> GGAGCGUCGUGUCUCUUGUACGUCUCGGUCACAAUACACGGUUUCGUCCGGUGCGUGGCAAUUCGGGGCACAUCAUGUCUUUCGUGGCUGGUGUGACCGCGCAAGGUGCGCGCGGUACGUAUCGAGCAGCGCUCC

Stem-loop 5 (SL5, residues 150 to 294) contains the start codon of open reading frame 1a/b (ORF1a/b, residues 266 to 268). Additionally, phylogenetic covariance analysis and chemical probing experiments have shown that SL5′s secondary structure forms a four-way junction that sequesters the genome’s start codon within one of its helical stems. Beyond SARS-CoV-2, the multi-way junction and the sequestration of the start codon in a stem are conserved features across most coronaviruses, despite large sequence divergence from SARS-CoV-2 (average sequence identity of 51% for the NCBI Reference Sequences for alpha- and betacoronaviruses). SL5 has been proposed to play a role in protein–RNA or RNA–RNA binding because of its conserved hexaloops, characterized by 5′-UUYYGU-3′ (Y = C, U) repeat loop motifs.

Expanding the cryo-EM analysis to more distant coronavirus relatives, we examined the orthologous SL5 domain from MERS (residues 206 to 338, 135 nt, 43.7 kDa), which belongs to the different Merbecovirus subgenus of betacoronaviruses. From the secondary structures obtained from large-library M2-seq and the literature, we already noted a difference: while the UUYYGU hexaloops are still found on SL5a and SL5b, the SL5c stem from MERS is significantly longer than SL5c from sarbecoviruses. Interestingly, our MERS SL5 cryo-EM analysis showed three conformations (6.9, 6.4, 6.4 Å resolution, 3.5, 3.2, 3.4 Å modeling convergence) and had the same conformation seen in sarbecovirus orthologs: helical stacking, junction geometry, and inter-helical angle matching within experimental error. While the four-way junction geometry is conserved between the sarbecovirus and merbecovirus orthologs, the merbecoviruses have a distinct ensemble of 3D folds that is conserved between MERS SL5 and BtCoV-HKU5 SL5. In particular, a flexible bend is observed emanating from the SL5a internal loop that allows the SL5a arm to swing in a hinge-like motion. To model this conformational heterogeneity, the particles were classified into discrete classes to resolve cryo-EM maps that could individually be modeled. Among these conformations, the junction geometry was conserved, with inter-helical angles occupying a narrow range of 81 to 84° and 84 to 88° for MERS and BtCoV-HKU5 SL5, respectively. Despite the junction geometry conservation, the relative locations of the hands of the SL5a and SL5b arms are variable due to the hinge in the SL5a internal loop, increasing the range of distance between UUYYGU hexaloops to 74 to 85 Å and 71 to 85 Å for MERS and BtCoV-HKU5 SL5, respectively. In addition, the merbecovirus orthologs display an unexpected tertiary interaction between the SL5a internal loop and SL5c apical loop, whereas the sarbecovirus SL5c stem is too short to form this tertiary interaction.> MIRAVFFDSLGTLISVEGAAKVHLKIMEEVLGDYPLNPKTLLDEYEKLAREAFSNYAGKPYRPLRDILEEVMRKLAEKYGFKYPENLWEISLRMAQRYGELYPEVVEVLKSLKGKYHVGVILNRDTEPATAFLDALGIKDLFDSITTSEEAGFFKPHPRIFELALKKAGVKGEKAVYVGDNPVKDAGGSKNL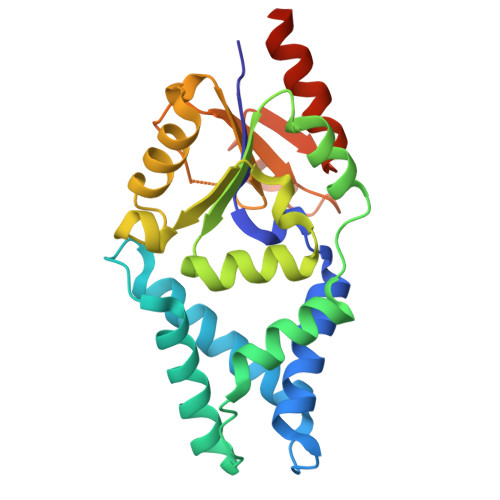GMTSILLDRKGEKREFWDKADFIVSDLREVIKIVDELNGQGSLEHHHHHH>[3x]AFIVNTNVPRA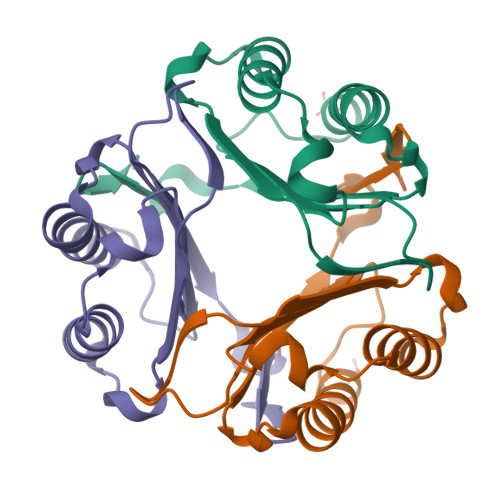SVPDGFLSELTQQLAQATGKPPQYIAVHVVPDQLMAFGGSSEPCALCSLHSIGKIGGAQNRSYSKLLCGLLAERLRISPDRVYINYYDMNAANVGWNNSTFA>MLDEKSSNTASVVVLATAPDEATAQDLAAKVLAEKLAAAATLIPGATSLYYWEGKLEQEYEVQMILKTTVSHQQALLEALKSHHPYQTPELLVLPVTHGDTDYLS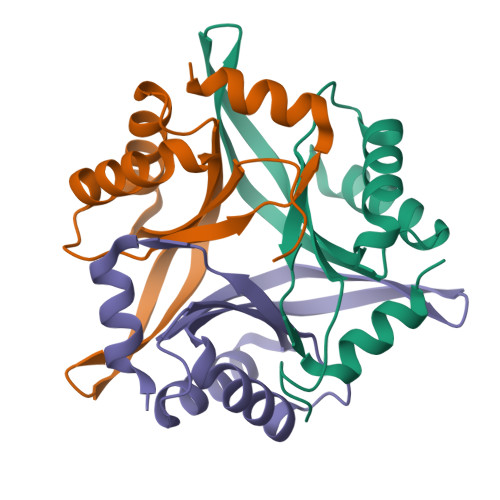WLNASLR[3x]> MLEETEAALLARVRELFGATLRQVEPLTGTWTNEDVHRLFLAPPSVFLAWMGCGEGRTRREVESRWAFFVVAELLNGEPVNRPGIYQIVERLIAGVNGQTFGPTTGMRLTQVRNLCDDNRINAGVVLYGVLFSGTTPLPSVVDLDSLDDYERHWQTWKFPDETPEF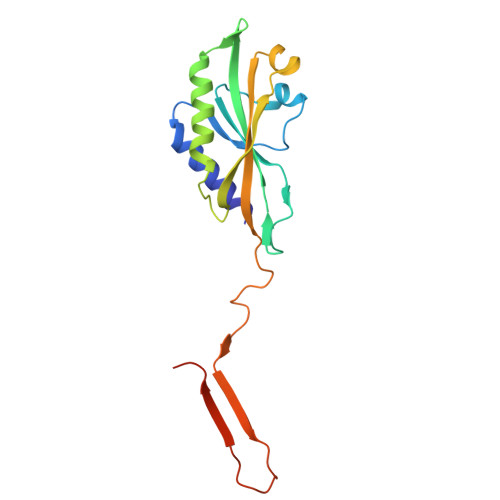AAHINVNQEKDHDAEN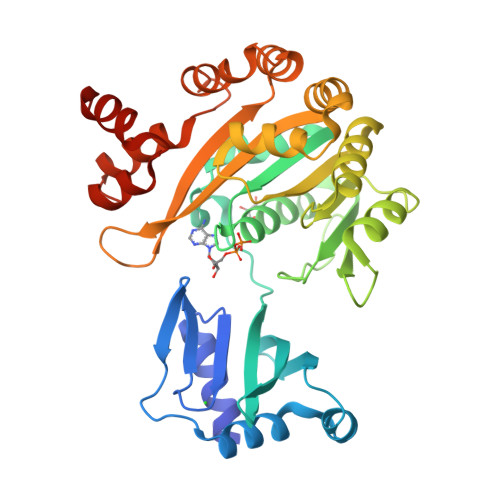> MSEAQGQGKQSLVEMLKAMVQARASDIHLQAGAPPTVRIDGKLRPFGNRPLTPKEVEAIARALLTPEQLEELEYRKEMDFAYTIPGVARFRCNLLRQRGSFGLVMRVVSEVIPSFEALGLPREVMESLAAKERGLILVTGPTGSGKSTTLAALIDHINLHYAKNIITIEDPIEFLHKHKKSLVVQREVGLDTDSFYTGLKYALRQDPDVIMVGEMRDRETVEAALMAAQTGHLVLSTLHTLDAWRTINRIIDFFPLHEHRQVRVLLAESLLGILSQRLLPKADGQGRVLALEILIATPYVRELLKDEEKTPQIKEAMMEGSLYGMRTFDQHLVELYTEGLISLEDALSAATSPHEFRLLLTKATGQTY> 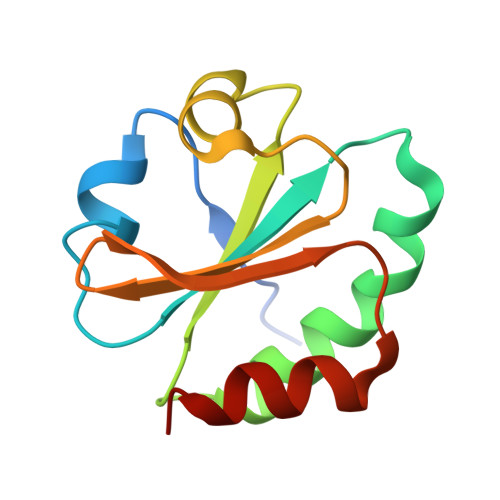CEAQETTTDIQVVNDSTWDSLVLKATGPVVVDFWAPWCGPSKMIDPLVNDLAQHYTGKIKFYKLNTDESPNTPGQYGVRSIPTIMIFVGGEKKDTIIGAVPKTTLTSSLDKFLP In this work, we have explored the structure and function of such non-insect OBPs in the mite Varroa destructor, a major pest of honey bee. Mass spectrometric analysis demonstrated that the six cysteines VdesOBPs, whose sequence position do not match the pattern in insect OBPs, are paired into three disulphide bridges (C1–C6, C2–C3 and C4–C5) different from that (C1–C3, C2–C5, C4–C6) of their insect counterparts. The overall folding, determined for VdesOBP1, is also novel and different from the conserved structure of insect OBPs, although some similar aspects can be recognised. Comparison with classical OBPs reveals that the second of the six α-helices found in them is lacking in VdesOBP1.

Another crystal form was collected, with space group P21 at 1.2 Å resolution, and its structure was determined by molecular replacement using the P3221 crystal form. VdesOBP1 crystal forms P3221 and P21 were crystallized at pH values of 7.5 and 9.5, respectively. They contain one and two molecules in the asymmetric unit, respectively. The chain was built in the electron density map of the P21 crystal form with the exception of residues 1–6 at the N-terminus, while the P3221 crystal form starts at residue 11 and lacks loop 50–53. In contrast, the P21 form contains two molecules in the asymmetric unit forming a crystallographic dimer. Finally, the PISA server reported an ambiguous response for the P21 form (score = 0.49) but discarded the possibility of a biological dimer in form P3221 (score = 0). The active site is empty, except in form P21 where a buffer molecule, 2-(N-cyclohexylamino)-ethane sulfonic acid (NCES), is docked against a wall of the binding site. Examination of the binding site in the crystallographic dimer revealed that the N-terminus of each monomer protrudes deeply in the binding site of the other monomer, drastically reducing its size. This effect explains the serendipitous binding of NCES as this ligand interacts with the cell wall of one monomer and the C-terminal extension of the other one.

>APQAPASATPAKVPVIEWGKCEQLKPSESERTSKAAVVDKCLQSLPLPDPEKATQQEIDKHRESVTTCALKAEGWFDDEGVYKFDRARNEIKNKKLDSEVEEAVLLKHDACQKEATEKHDDYINQVQLYQACMDYNISQICGIKVMV[2x]> MKKVSSFKLGMVLLLIAAVCGLILGGVNQVTAEPIAI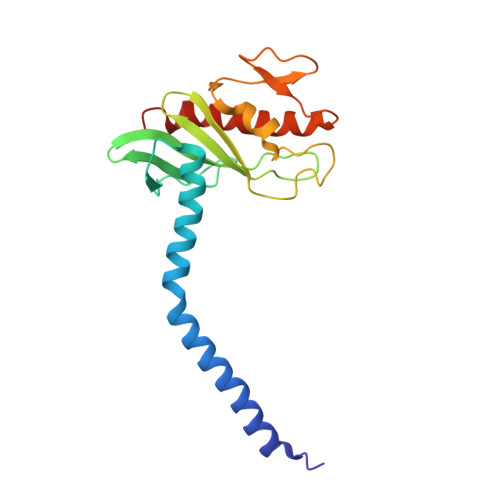QNKKTLDEANKAILPEASEFAEKTDIKGEGIVLGVTEGKSGSDLKGYTIKVAPKGYAGAIEMMVGVSTEGKVTGIKILNHAETPGLGANATDPKFSGQYANKPAKELKVVKGAASGEDEIVAITGATITSKAVTLGVNEAIKFYDTKLKGGK>GAMALYEFVGLLDAHGNVLEVNQVALEGGGITLEEIRGK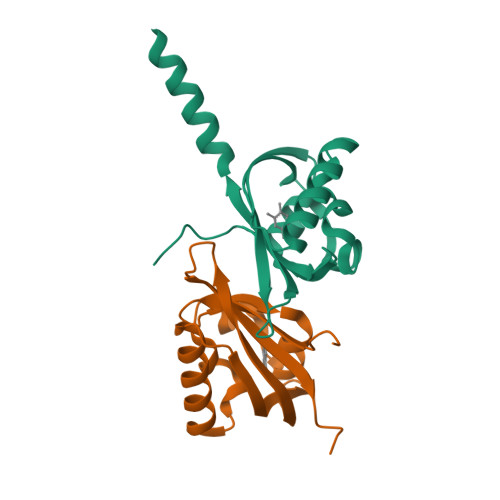PFWKARWWQISKKTEATQKRLVETASSGEFVRCDVEILGKSGGREVIAVDFSLLPICNEEGSIVYLLAEGRNITDKKKAEAMLALKNQELE[2x]>[3x]MQEITVDEFSNIRENPVTPWNPEPSAPVIDPTAYIDPEASVIGEVTIGANVMVSPMASIRSDEGMPIFVGDRSN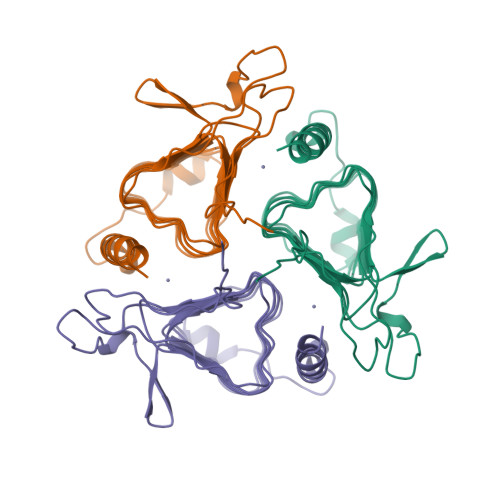VQDGVVLHALETINEEGEPIEDNIVEVDGKEYAVYIGNNVSLAHQSQVHGPAAVGDDTFIGMQAFVFKSKVGNNCVLEPRSAAIGVTIPDGRYIPAGMVVTSQAEADKLPEVTDDYAYSHTNEAVVYVNVHLAEGYKETS N6-benzyl-(alpha,beta)-methylene-ADP | C18 H23 N5 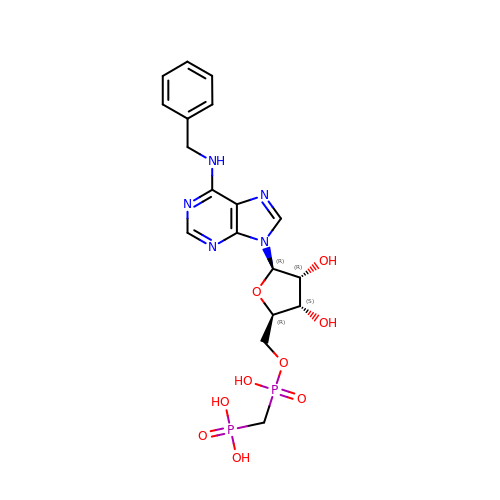O9 P2 | DMBYYIJBPDWQFF-SCFUHWHPSA-N>[6x]MGYFELQLSALRNVNGELLSGACCDGDGRTTRAGGCGHDECDTYVRVCLKEYQAKVTPTGPCSYGHGATPVLGGNSFYLPPAGAAGDRARARARAGGDQDPGLVVIPFQFAWPRSFTLIVEAWDWDNDTTPNEELLIERVSHAGMIN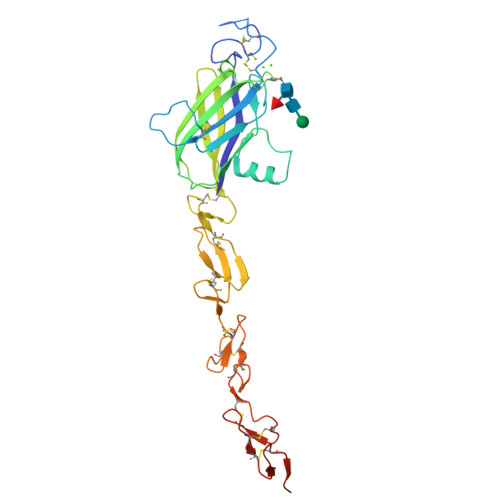PEDRWKSLHFSGHVAHLELQIRVRCDENYYSATCNKFCRPRNDFFGHYTCDQYGNKACMDGWMGKECKEAVCKQGCNLLHGGCTVPGECRCSYGWQGRFCDECVPYPGCVHGSCVEPWQCNCETNWGGLLCDKDLNGSHHHHHHHH2-[hydroxy(4-hydroxybutyl)amino]-2-oxoethyl dihydrogen phosphate | C6 H14 N O7 P | 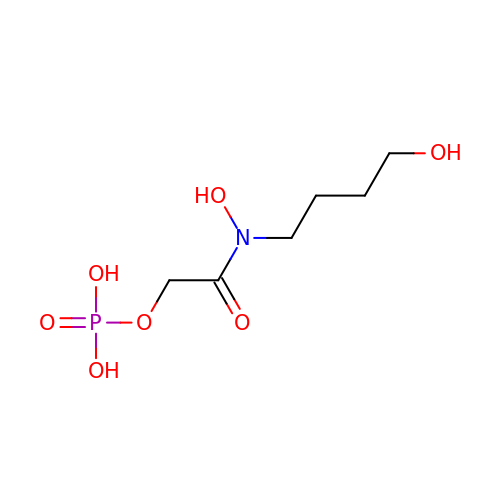XYJLIJWOOPZDNB-UHFFFAOYSA-N> TVAYIAIGSNLASPLEQV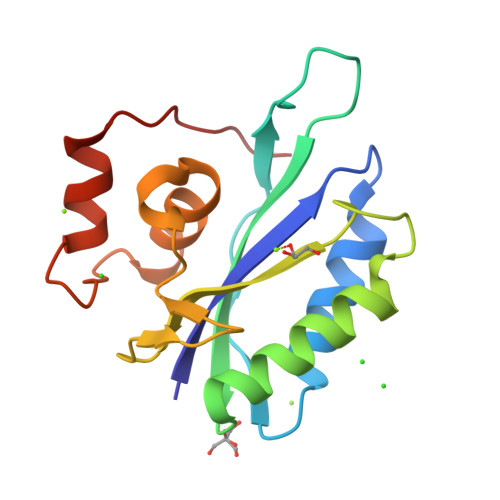NAALKALGDIPESHILTVSSFYRTPPLGPQDQPDYLNAAVALETSLAPEELLNHTQRIELQQGRGGPRTLDLDIMLFGNEVINTERLTVPHYDMKNRGFMLWPLFEIAPELVFPDGEMLRQILHTRAFDKLNKW>SMVTIKVFSPKYPTELEEFYAERIADNPLGFIQRLDLLPSISGFVQKLREHGGEFFEMREGNKLIGICGLNPINQTEAELCKF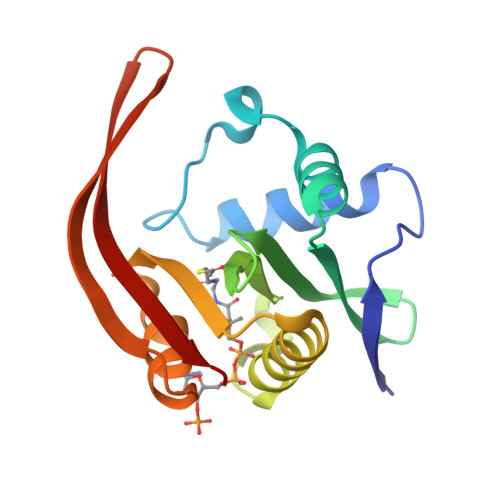HINSAYQSQGLGQKLYESVEKYAFIKGYTKISLHVSKSQIKACNLYQKLGFVHIKEEDCVVELGEETLIFPTLFMEKILS[4x]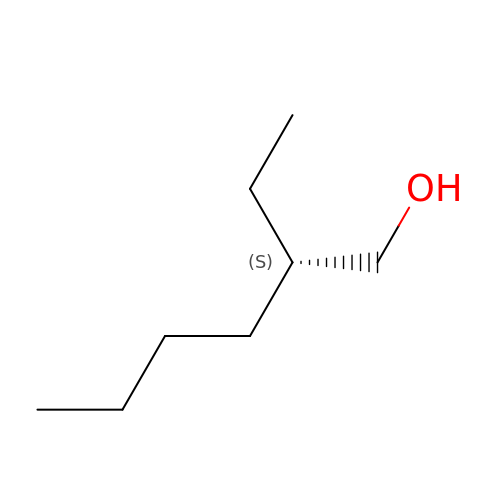(2S)-2-ethylhexan-1-ol | C8 H18 O | YIWUKEYIRIRTPP-QMMMGPOBSA-N1-[(3-methyl-1-{2-[(1-methyl-1H-indazol-5-yl)amino]pyrimidin-4-yl}-1H-pyrazol-4-yl)methyl]azetidin-3-ol | C20 H22 N8 O | 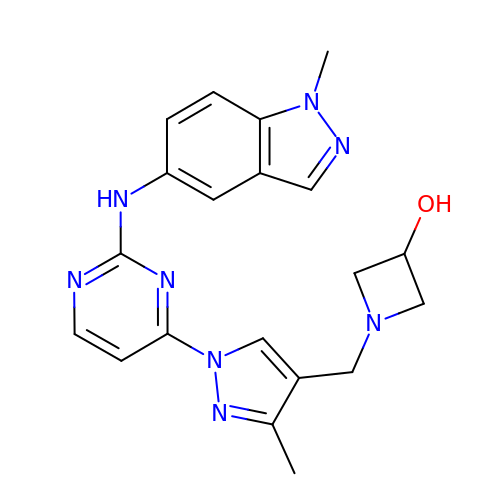FFTGDASJRVPWKO-UHFFFAOYSA-N> MLKKLFGAKKEFYVQLDESQAPAQVE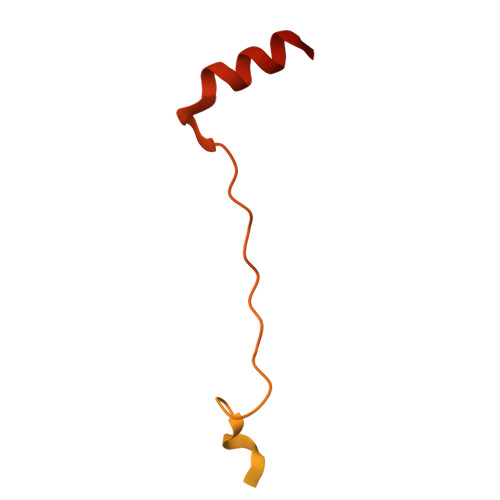EADVAIVKSEVAPVEKPAPTTSKKTSIKKKSATKAAAPVETPASAPVAPAPKAKVDPSQVAFASGDPIPQNVARRTPGPSLNRFKEMARQVKVKR{[(2R)-2-[(2-amino-6-oxo-1,6-dihydro-9H-purin-9-yl)methyl]-3-(2-phosphonoethoxy)propoxy]methyl}phosphonic acid | C12 H21 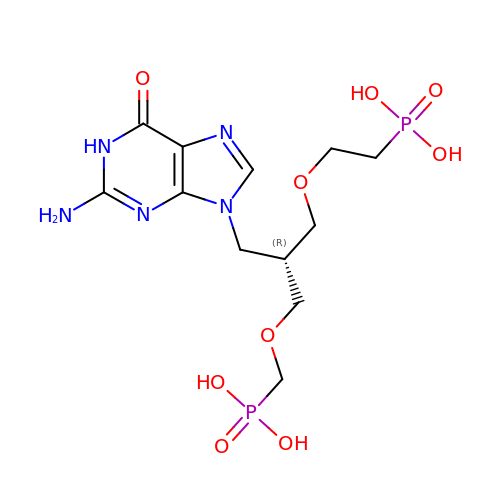N5 O9 P2 | VTOAZXSSULBZBZ-MRVPVSSYSA-N> MEARAHGALPNNYDRERFINGVGGDDKALKRKLEEPLSDITKELDTVIAQSDVAVADPKGQLCPDADVPDEMEHITDGILPLNLLLIRLAEFSHSKLEELVTMLASKPVPQHAVNGNGSHSTLVEDASPESQEKKRLLLNTIQDLHSRWVKALVITEWARNAEKVGKLIDIRTHLFKKLELYPQVLNDFINLKRDMAWAKVPSPDLKTALHILTHGEVTWMPDFNFLDPPPLTTEETLRWINDMNLALHARLQLEEHDKLPPPFKNYTIDSGRVTFRVRGEFEVDLSISEEDFSEQFWFINFRFDFSPAPAELTPAVRYWMTEKVNNILKTEGLGGCYKYLH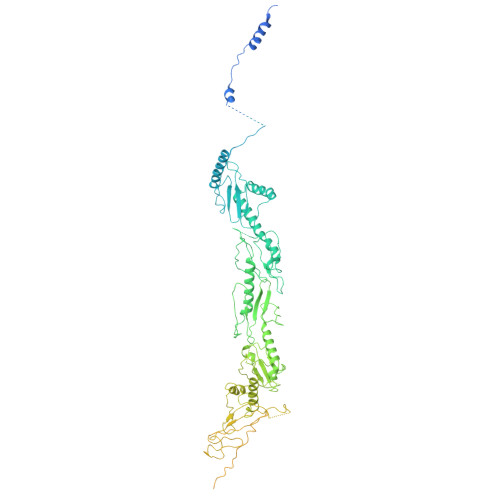EFTLTQKIAELHRQAIALNKGRWANSLRVEKLNRNLGIHYWANRLHSQNLKSWIIIGVHSGEDPQGLEEPKPSYLMVQWFREGVEQFIDIPFSQEKLSIEEILEFVTAKHVGYLLFSLFRKFDGKPRFTQGKKARLELNVWTQKPEDYYLSMQLLDDEDLKIQVNPWMGDFITTPSTGPWNRTLNSLGNPAEEGSKELENFRYIYIISVLKAQGKSHGWSVVRSPISQDELRSIVHSESASSRETFQAAWTRFVDWDPQWYAMRSMSLAGDQWWLVEVTSQRQSISGNRLVFFTKMAPCFSEERLTDGFFNGLRDHSRRLIAEITNLRELYPGITPSQLRKLIDPTRQPPVLPVKASKILGDFGGADAQSIAWLKDPVWLIYRGSACDAAATRVSDSPQQKRTQPVLDVFEAYLDVTDRRRFQTLNPRLDRDILYNPYTGRFMFRLRAKMGVPVVPLLGIRVRQLQRLLDFLEGLRRVGDQAVPERVTLREIVFSYGATRKRDSTNQPKVRPWRVRLDLTKEEGVGVVLEKGNPHLRVINRLEDLVNSQKFYSLATYLTLSLPLFRAFEQLENAWQTAQENGRGSCFILHLSLDKHTIRFVLPGHQRQISLLIQPHEKEGKLVWEVGRPRHDPELLNENCEFNRVLKERVWTISGSGFKGLVTGAAAEPDEGIERLLVLISDAVLHLSTSQPATAPPQPPQAQPSQQVQQVQQQQVVSQLQPQAQQPRSAMPHASVGQQQPHGAPAPMARFPPQQQQIFQQQRPPQPQPNMHGGQISQPNMHGGPKPQLQGQHGQPGQMVAAPQQQGQRPGTGTAAGMGRSNAPLVVLD> SDFANLSSTNKELS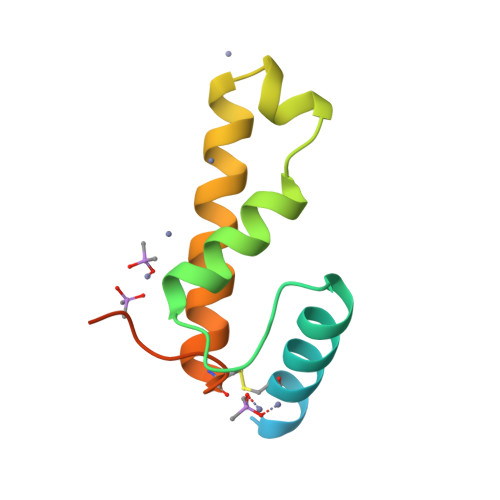PQYNWVACGILEGGLKAAGVLEEGQYNRELAEAIAAKGEGFWTTQFPQIGDWNEDQAAALADRAQTCGLVKADTYLSELSSNFSS> GSHMASPNGQTKPLPALKLALEYIVPCMNKHGICVVDDFLGKETGQQIGDEVRALHDTGKFTDGQLVSQKSDSSKDIRGDKITWIEGKEPGCETIGLLMSSMDDLVLHCNGKLGSYKVNGRTKAMVACYPGNGTGYVRHVDNPNGDGRCVTCIYY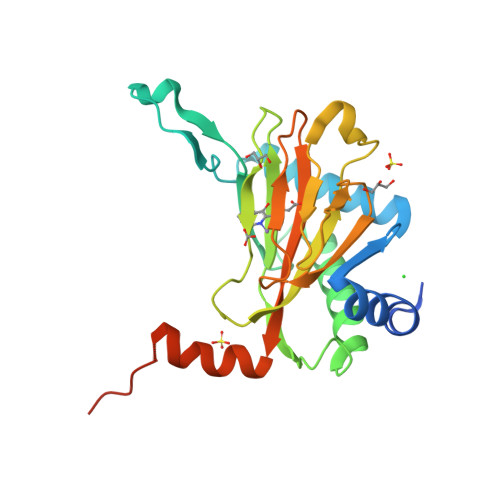LNKDWDAKVSGGILRIFPEGKAQFADIEPKFDRLLFFWSDRRNPHEVQPAYATRYAITVWYFDADERARAKVKYLTGEKGVRVELNKPSDSVGKDVF>[2x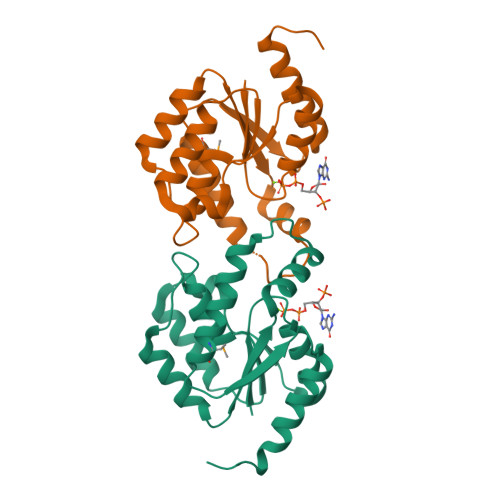]MTLIILEGPDCCFKSTVAAKLSKELKYPIIKGSSFELAKSGNEKLFEHFNKLADEDNVIIDRFVYSNLVYAKKFKDYSILTERQLRFIEDKIKAKAKVVYLHADPSVIKKRLRVRGDEYIEGKDIDSILELYREVMSNAGLHTYSWDTGQWSSDEIAKDIIFLVELEHHHHHH Each system consists of a Tandem Interspaced Guide RNA (TIGR) array and a TIGR-associated (Tas) protein containing a Nop domain, sometimes fused to HNH (TasH) or RuvC (TasR) nuclease domains. We show that TIGR arrays are processed into 36-nt RNAs (tigRNAs) that direct sequence-specific DNA binding through a tandem-spacer targeting mechanism. TasR can be reprogrammed for precise DNA cleavage, including in human cells. The structure of TasR reveals striking similarities to box C/D snoRNPs and IS110 RNA-guided transposases, providing insights into the evolution of diverse RNA-guided systems.

The TasR dimer binds one copy of the target DNA and one copy of the 36-nt tigRNA. The cryo-EM density shows clear discontinuity at the expected cleavage position on both target DNA strands, consistent with the cryo-EM reconstruction capturing a product state, and each TasR RuvC domain active site is positioned in close proximity to each nick, with four highly conserved acidic residues located near the catalytic magnesium ion. The DNA substrate undergoes a dramatic 180° turn as it enters and exits the complex. The 18-bp target sequence itself is unwound, whereas all flanking sequences are fully base-paired in canonical B-form helices that do not form any base-specific interactions with the TasR protein or tigRNA, consistent with the lack of a targeting motif. All 9 nt of the spacer A-complementary strand are paired with tigRNA spacer A, forming an A-form helix, whereas the non-complementary strand is single stranded and is separated from its complementary strand by a ‘wedge loop’ insertion domain of the TasR protein. Spacer B and the spacer-B complementary strand are recognized in an identical manner. The minor groove of the tigRNA/DNA duplex rests on the TasR coiled-coil dimerization domain, and notably, the two base pairs that we identified as the ‘seed’ region make the closest interactions with the coiled coil, suggesting that the coiled-coil domain could increase fidelity by probing for correct helix geometry at the seed positions. The 36-nt tigRNA forms a pseudosymmetric figure-eight shape as it interacts with both TasR protomers and both DNA target strands. Once accounting for the pseudosymmetry, we observed that the edge repeat interacts with the Nop domain of one TasR protomer, whereas the loop repeat makes almost identical interactions with the other protomer. To determine the precise sites of DNA cleavage by TasR, we used Sanger sequencing and found that each spacer specified the nicking site in an identical way, with each strand cut 3′ to the nucleotide complementary to the 5th base of the spacer, resulting in a double-strand break with 8-nt 3′ overhangs.

>[2x]MDNDITILAVDWSHEERKLAIFDGKKIRKKLPEPSSDVIIVAENIPQKYAAPFIEVGAKVLRCSTNATADARKNYQKKVDAAFAKNDENDSKVIWALYQTHPELFREMKLEPPLSSYYAIFKDYQEVRIRTGNRLYSDRTDAMEEFFKIVKKGEHELKKAVDKELENHPVYTQWLQHIKGIGPVVAGGLISLIGDIDRFDSVSKLWAYAGYSVDNGKVQKRKKGVASNWKNKIRTHCYNIVDSFIKQRTSVYRELYDAEKARQRPKVESDGHAHNRAVRKVAKVFLQHYWVVSRELAGFSVSKPWILEHGGHVDYIKPPHWNKVEIKPCKP> HTTEAEASSQSLTQIYAL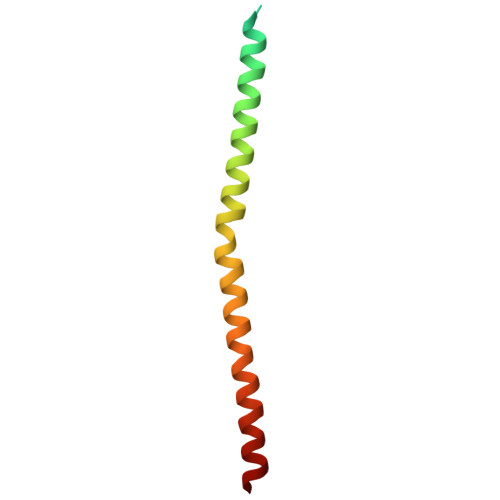PEIPQDQNAAESWETLEADLIELSQLVTDFSLLVNSQQEKIDSIADHVNSAAVNVEEGTKNLGKAAKYK>GAMDIAAQAKLVYHLNKYYNEKCQARKAAIAKTIREVCKVVSDVLKEVEVQEPRFISSLNEMDNRYEGLEVISPTEFEVVLYLNQMGVFNFVDDGSLPGCAVLKLSDGRKRSMSLWVEFITASGYLSARKIRSRFQTLVAQAVDKCSYRDVVKMVADTSEVKLRIRDRYVVQITPAFKCTGIWPRSAAHWPLPHIPWPGPNRVAEVKAEGFNLLSKECHSLAGKQSSAESDAWVLQFAEAENRLQMGGCRKKCLSILKTLRDRHLELPGQPLNNYHMKTLVSYECEKHPRESDWDESCLGDRLNGILLQLISCLQCRRCPHYFLPNLDLFQGKPHSALENAAKQTWRLAREILTNPKSLEKL[10x]

The male abnormal 21 (MAB21) like proteins form a sequence related subfamily within the large and diverse family of nucleotidyltransferase (NTase) fold proteins. Here, we provide the first crystal structure of a MAB21 protein and the structure of MAB21L1 bound to CTP. MAB21L1 is a two lobed, globular protein of a mixed α/β topology with approximate molecular dimensions of 64 Å × 35 Å × 48 Å. The human MAB21L1 structure exhibits a high degree of structural conservation with cGAS but features a number of differences.

To further address the nucleotide binding, we co-crystallized MAB21L1 with both ATP and CTP in the crystallization condition and determined the resulting crystal structure of MAB21L1 to 2.55 Å resolution. In this structure each protomer shows clear density for a single CTP moiety, and we did not see any density for ATP. Unexpectedly, the CTP moiety is not localized at the NTase active site, but rather bound at the positively-charged pocket on the ‘platform’ side of the molecule adjacent to the spine helix. In the loop connecting α1-β1, R62 stacks with the cytosine base in a planar conformation. This loop is better resolved in the MAB21L1:CTP structure, compared to apo MAB21L1, arguing for some sort of induced fit. Backbone interaction between L66 and Y63 and the amino group at C4 of the cytosine explain the preference of MAB21L1 for CTP and ATP, compared to UTP and GTP where no binding affinity was detected. The α-phosphate is coordinated by K255 and R23, the β-phosphate builds salt bridges with K255 and S252 and R23, while the γ-phosphate is held in place by K24 and K248. In summary, CTP binding did not obviously affect the overall conformation of MAB21L1 and the superposition of apo MAB21L1 (crystallized without added nucleotides) and MAB21L1 in complex with CTP reveals no major conformational changes (RMSD 0.94 Å). CTP binding to MAB21L1 appears to stabilize the current, presumably inactive, conformation. Obviously CTP did not switch the protein into an active conformation, so CTP is unlikely a physiological activating ligand.>[4x]NAMPPIIKRRVMRKIIIASQNPAKVNAVRSAFSTVFPDQEWEFIGVSVPSEVADQPMSDEETKQGALNRVRNAKQRHPG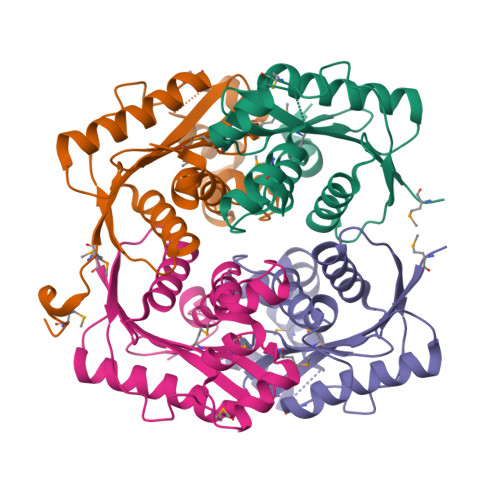AEYYVGLEAGIEENKTFAWMIVESDQQRGESRSACLMLPPLVLERLRQAKELGDVMDEVFGTENIKQKGGAIGLLTRHHLTRSTVYHQALILALIPFINPEHYPSA>MPCSEETPAISPSKRARPAEVGGMQLRFARLSEHATAPTRGSARAAGYDLYSAYDYTIPPMEKAVVKTDIQIALPSGCYGRVAPRSGLAAKHFIDVGAGVIDEDYRGNVGVVLFNFGKEKFEVKKGDRIAQLICERI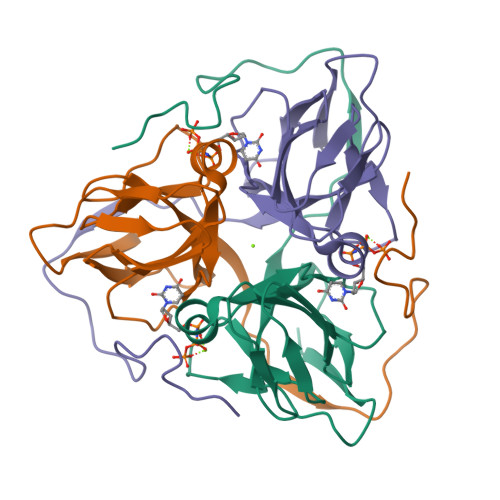FYPEIEEVQALDDTERGSGGFGSTGKN[6x]>[2x]MYGLVNKAIQDMISKHHGEDTWEAIKQKAGLEDIDFFVGMEAYSDDVTYHLVGAASEVLGKPAEEL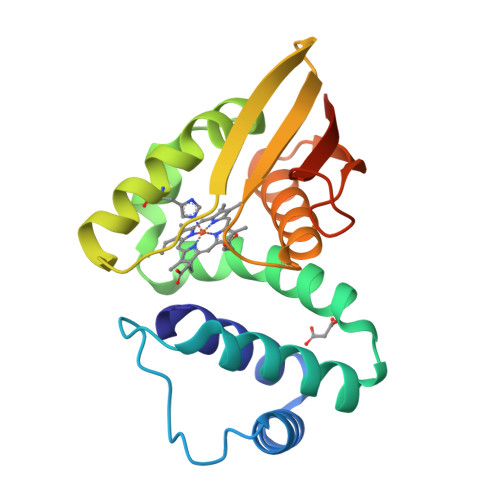WIAFGEYWVTYTSEEGYGELLASAGDSLPEFMENLDNLHARVGLSFPQLRPPAFECQHTSSKSMELHYQSTRCGLAPMVLGLLHGLGKRFQTKVEVTQTAFRETGEDHDIFSIKYEDSNLYDD>MHHHHHHHLEAPSPYSTLVVFGDSLSDAGQFPDPAGPAGSTSRFTNRVGPTYQNGSGEIFGPTAPMLLGNQLGIAPGDLAASTSPVNAQQGIADGNNWAVGGYRTDQIYDSITAANGSLIERDNTLLRSRDGYLVDRARQGLGADPNALYYITGGGNDFLQGRILNDVQAQQAAGRLVDSVQALQQAGARYIVVWLLPDLGLTPATFGGPLQPFASQLSGTFNAELTAQLSQAGANVIPLNIPLLLKEGMANPASFGLAADQNLIGTCFSGNGCTMNPTYGINGSTPDPSKLLFNDSVHPTITGQRLIADYTYSLLSAPWELTLLPEMAHGTLRAYQDELRSQWQADWENWQNVGQWRGFVGGGGQRLDFDSQDSAASGDGNGYNLTLGGSYRIDEAWRAGVAAGFYRQKLEAGAKDSDYRMNSYMASAFVQYQENRWWADAALTGGYLDYDDLKRKFALGGGERSEKGDTNGHLWAFSARLGYDIAQQADSPWHLSPFVSADYARVEVDGYSEKGASATALDYDDQKRSSKRLG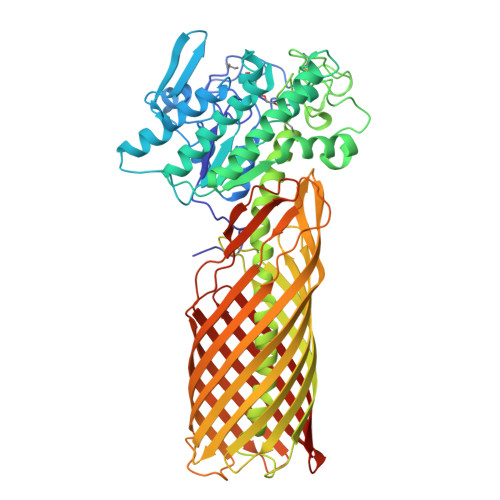AGLQGKYAFGSDTQLFAEYAHEREYEDDTQDLTMSLNSLPGNRFTLEGYTPQDHLNRVSLGFSQKLAPELSLRGGYNWRKGEDDTQQSVSLALSLDF[2x]> MVANQANLIDNKRELEQHALVPYAQGKSIHQLFEEQAEAFPDRVAIVFENRRLSYQELNRKANQLARALLEKGVQTDSIVGVMMEKSIENVIAILAVLKAGGAYVPIDIEYPRDRIQYILQDSQTKIVLTQKSVSQLVHDVGYSGEVVVLDEEQLDARETANLHQPSKPTDLAYVIYTSGTTGKPKGTMLEHKGIANLQSFFQNSFGVTEQDRIGLFASMSFDASVWEMFMALLSGASLYILSKQTIHDFAAFEHYLSENELTIITLPPTYLTHLTPERITSLRIMITAGSASSAPLVNKWKDKLRYINAYGPTETSICATIWEAPSNQLSVQSVPIGKPIQNTHIYIVNEDLQLLPTGSEGELCIGGVGLARGYWNRPDLTAEKFVDNPFVPGEKMYRTGDLAKWLTDGTIEFLGRIDHQVKIRGHRIELGEIESVLLAHEHITEAVVIAREDQHAGQYLCAYYISQQEATPAQLRDYAAQKLPAYMLPSYFVKLDKMPLTPNDKIDRKALPEPDLTANQSQAAYHPPRTETESILVSIWQNVLGIEKIGIRDNFYSLGGDSIQAIQVVARLHSYQLKLETKDLLNYPTIEQVALFVKSTTRKSDQGIIAGNVPLTPIQKWFFGKNFTNTGHWNQSSVLYRPEGFDPKVIQSVMDKIIEHHDALRMVYQHENGNVVQHNRGLGGQLYDFFSYNLTAQPDVQQAIEAETQRLHSSMNLQEGPLVKVALFQTLHGDHLFLAIHHLVVDGISWRILFEDLATGYAQALAGQAISLPEKTDSFQSWSQWLQEYANEADLLSEIPYWESLESQAKNVSLPKDYEVTDCKQKSVRNMRIRLHPEETEQLLKHANQAYQTEINDLLLAALGLAFAEWSKLAQIVIHLEGHGREDIIEQANVARTVGWFTSQYPVLLDLKQTAPLSDYIKLTKENMRKIPRKGIGYDILKHVTLPENRGSLSFRVQPEVTFNYLGQFDADMRTELFTRSPYSGGNTLGADGKNNLSPESEVYTALNITGLIEGGELVLTFSYSSEQYREESIQQLSQSYQKHLLAIIAHCTEKKEVERTPSDFSVKGLQMEEMDDIFELLANRLRGSRSHHHHHH;> MGVFSKEQVQDMYALTPMQEGMLFHALLDQEHNSHLVQMSISLQGDLDVGLFTDSLHVLVERYDVFRTLFLYEKLKQPLQVVLKQRPI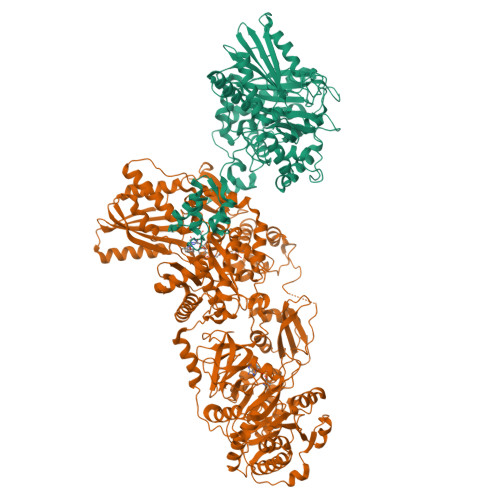PIEFYDLSACDESEKQLRYTQYKRADQERTFHLAKDPLMRVALFQMSQHDYQVIWSFHHILMDGWCFSIIFDDLLAIYLSLQNKTALSLEPVQPYSRFINWLEKQNKQAALNYWSDYLEAYEQKTTLPKKEAAFAKAFQPTQYRFSLNRTLTKQLGTIASQNQVTLSTVIQTIWGVLLQKYNAAHDVLFGSVVSGRPTDIVGIDKMVGLFINTIPFRVQAKAGQTFSELLQAVHKRTLQSQPYEHVPLYDIQTQSVLKQELIDHLLVIENYPLVEALQKKALNQQIGFTITAVEMFEPTNYDLTVMVMPKEELAFRFDYNAALFDEQVVQKLAGHLQQIADCVANNSGVELCQIPLLTEAETSQLLAKRTETAADYPAATMHELFSRQAEKTPEQVAVVFADQHLTYRELDEKSNQLARFLRKKGIGTGSLVGTLLDRSLDMIVGILGVLKAGGAFVPIDPELPAERIAYMLTHSRVPLVVTQNHLRAKVTTPTETIDINTAVIGEESRAPIESLNQPHDLFYIIYTSGTTGQPKGVMLEHRNMANLMHFTFDQTNIAFHEKVLQYTTCSFDVCYQEIFSTLLSGGQLYLITNELRRHVEKLFAFIQEKQISILSLPVSFLKFIFNEQDYAQSFPRCVKHIITAGEQLVVTHELQKYLRQHRVFLHNHYGPSETHVVTTCTMDPGQAIPELPPIGKPISNTGIYILDEGLQLKPEGIVGELYISGANVGRGYLHQPELTAEKFLDNPYQPGERMYRTGDLARWLPDGQLEFLGRIDHQVKIRGHRIELGEIESRLLNHPAIKEAVVIDRADETGGKFLCAYVVLQKALSDEEMRAYLAQALPEYMIPSFFVTLERIPVTPNGKTDRRALPKPEGSAKTKADYVAPTTELEQKLVAIWEQILGVSPIGIQDHFFTLGGHSLKAIQLISRIQKECQADVPLRVLFEQPTIQALAAYVELEHHHHHH Nevertheless, the tri-Asp site in LarE represents an unusual metal binding site that selectively and stoichiometrically binds certain multivalent cations. In the apoprotein structure the tri-Asp site is pre-formed to receive a metal ion by a hydrogen bond network consisting of Asp231, Arg228, Gly207, and several water molecules filling the site. Notably, the arginine residues form a positively charged ring around the tri-Asp site, limiting the metal-Asp interactions along the three-fold symmetry axis and likely responsible for only one metal ion being captured by these residues. We observed binding to the tri-Asp site for Ca2+, Mn2+, both Fe2+ and Fe3+, Co2+, Ni2+, Cu2+, Zn2+, and Cd2+, whereas Mg2+, K+, Cr3+, Cu+ and Cs+ did not bind at that location (data not shown).

In all cases, the Asp231 side chains bind the metals with bidentate coordination, with a seventh site always showing extra density that we modelled as a water molecule. Even in the case of the low resolution Co2+ bound dataset this extra density is observed. As 3.55 Å dataset resolution cannot justify placement of water alone we inferred the shown mode based on the observations in the other datasets. In general, soaking experiments reduced diffraction power and had a negative effect on merging statistics; especially the Cu and Co datasets were of worse quality than the apoprotein datasets or those for other metals like Ca. Several metal soaks (Co, Ni, Zn, and Cd) also resulted in binding of these metals to surface exposed residues. These partially disordered sites only appeared after metal soaks, showing a significant electron density peak and in some cases anomalous peaks. In most cases the surface site involved only a single histidine residue. This resulted in higher B-factors of these metals compared to the tri-Asp site. For small molecule complexes in the Cambridge Structural Database (CSD) the most common and second most frequent coordination numbers for Mn2+, Fe2+/3+, Co2+, Ni2+, Zn2+, and Cd2+ are 6 and 4; while for Ca2+ they are 6 and 7; and for Cu2+ they are 5 and 635. We reason that the tri-Asp site captures low levels of contaminating metal ions, most likely Ni, Co, or Cd, from the Superdex 200 resin used for other protein purifications in the laboratory.

>MATLATKKATLVAALKDLQRVTVAFSGGIDSTLVLKMALDVLGRDNVTAVVANSELFTDEEFDKAMSLAEELGANVQGTTLDYLSDDHIKNNTPDSWYYAKKMFYSRLNDIAANNGSAAVLDGMIKNDENDYRPGLKARSEAGARSLLQEADFFKTDVRALAQELGLTNWNKVASCSVSSRFPYGTTLTHDNIAQVMAAEKYLRSLGFPTVRVRFHNDIARIELPEARIGDFLVFNDRVNRQLQSLGFRYVTLDLGGFRSGRMNDTLTKAQLATFAASWSHPQFEK[6x]1-TER-BUTYL-3-P-TOLYL-1H-PYRAZOLO[3,4-D]PYRIMIDIN-4-YLAMINE 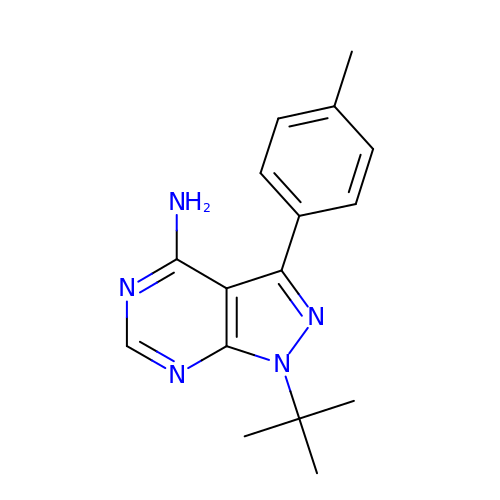| C16 H19 N5 | ZVPDNRVYHLRXLX-UHFFFAOYSA-N>MDSKQQCVKLNDGHFMPVLGFGTYAPPEVPRSKALEVTKLAIEAGFRHIDSAHLYNNEEQVGLAIRSKIADGSVKREDIFYTSKLWSTFHR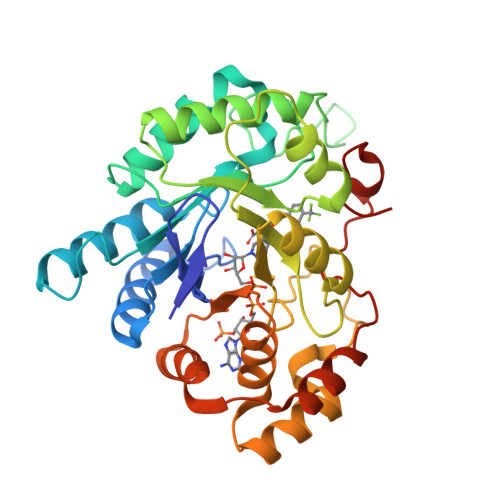PELVRPALENSLKKAQLDYVDLYLIHSPMSLKPGEELSPTDENGKVIFDIVDLCTTWEAMEKCKDAGLAKSIGVSNFNRRQLEMILNKPGLKYKPVCNQVECHPYFNRSKLLDFCKSKDIVLVAYSALGSQRDKRWVDPNSPVLLEDPVLCALAKKHKRTPALIALRYQLQRGVVVLAKSYNEQRIRQNVQVFEFQLTAEDMKAIDGLDRNLHYFNSDSFASHPNYPYSDEY[2x]>[3x]STKKKPLTQEQLEDARRLKAIYEKKKNELGLS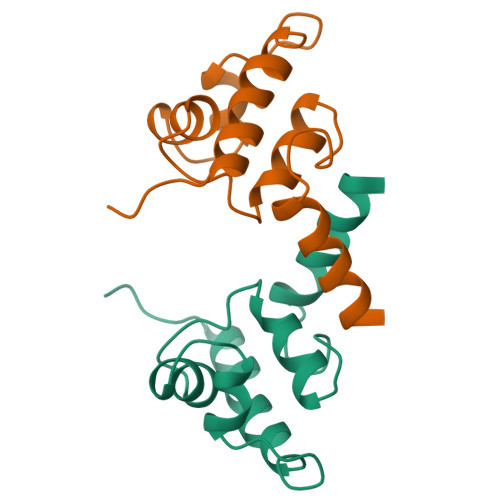QESVADKMGMGQSGVGALFNGINALNAYNAALLAKILKVSVEEFSPSIAREIYEMYEAVS> RPQGATVSLWETVQKWREYRRQCQRSLTEDPPPATDLFCNRTFDEYACWPDGEPGSFVNVSCPWYLPWASS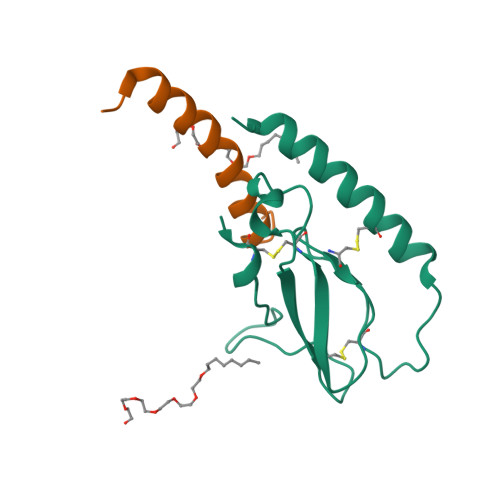VPQGHVYRFCTAEGLWLQKDNSSLPWRDLSECEESKRGERSSPEEQLLFLY;> HAEGTFTSDVSSYLEGQAAKEFIAWLVRGRG>MDFPLANLFFVPSEDATAFGRRLRAAAQQAPIVFDTAFGMPILLRKSHITTAYRDTATFSTRMFQAGILNGGLAAMQGDEHARMRRVYNMFFLPRAVSQYEERFVRPISEQVVDRLAGKPRVDLLEDFAMELPRRVIGELFGFPAEKLHETDERVRAMLRGLVRMHDPAAVAESQRAYGETLGLITEVVERESRDTSDTLLGEILRTLKAEHMDTIEASRQIVLSLILGGYETTSWLVANTIHALLAHPDTLARVRQDPSLLPAAIEEGMRWCPSIFGVLRMVERDVRLDDQALSAGTVVC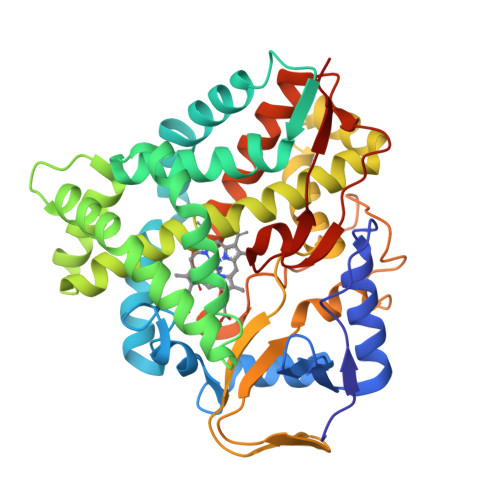LAGIAGNYDETAYPSPEVYDIDRKPLPAANVFGGGAHFCVGAPLARMEARVGLQALLARFPGLRAVPEERPSFMYGAKDSVAHGPDKLPVLLHHHHHHH[2x]>SGSPTPLETLPLEELERRALKIYLRRHGSVPEEEIETMPLEELERKALQDYLRRYGTLPEEEIETMPLEELEREALKNYLRRYGTLPEEEIDT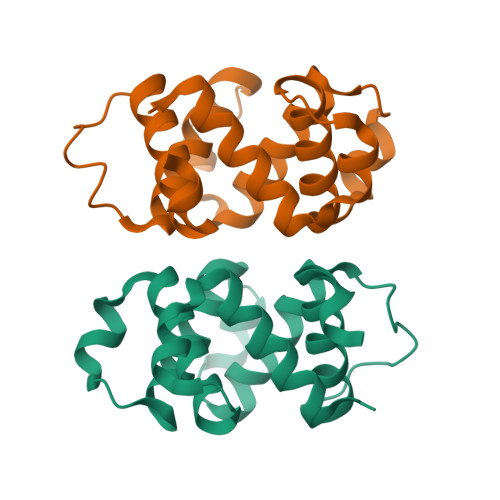MPLEELEREALKNYLRRYGSLPPEELEKLPLEELERKALIEYLRRYGPSGSG[2x]> MLEPLRLSQLTVALDARLIGEDAVFSAVSTDSRAIGPGELFIALSGPRFDGHDYLAEVAAKGAVAALVEREVADAPLPQLLVRDTRAALGRLGALNRRKFTGPLAAMTGSSGKTTVKEMLASILRTQAGDAESVLATRGNLNNDLGVPLTLLQLAPQHRSAVIELGASRIGEIAYTVELTRPHVAIITNAGTAHVGEFGGPEKIVEAKGEILEGLAADGTAVLNLDDKAFDTWKARASGRPLLTFSLDRPQADFRAADLQRDARGCMGFRLQGVAGEAQVQLNLLGRHNVANALAAAAAAHALGVPLDGIVAGLQALQPVKGRAVAQLTASGLRVIDDSYNANPASM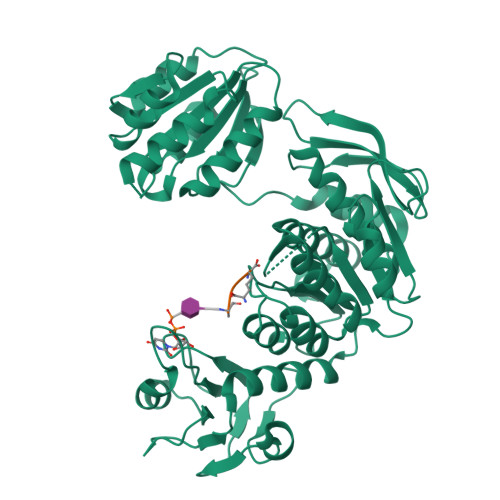LAAIDILSGFSGRTVLVLGDMGELGSWAEQAHREVGAYAAGKVSALYAVGPLMAHAVQAFGATGRHFADQASLIGALATEDPTTTILIKGSRSAAMDKVVAALCGSSEESHSSVDKLAAALEHHHHHH;> AEK N-(6-chloro-1,3-benzothiazol-2-yl)-1-benzothiophene-2-sulfonamide 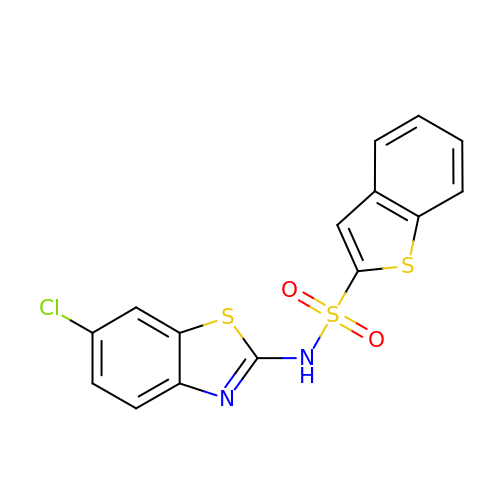| C15 H9 Cl N2 O2 S3 | MZAVPBQCWWIYEQ-UHFFFAOYSA-N>ADYVLAIDQGTTSSRAIVFDHSGEIYSTGQLEHDQIFPRAGWVEHNPEQIWNNVREVVGLALTRGNLTHEDIAAVGITNQRETAVVWDKTTGKPVYNAIVWQDTRTQKIVDELGGDEGAEKYKSIVGLPLATYFSGPKIKWILDNVEGAREKAEKGDLLFGNTDTWVLWNMTGGTEGGVHVTDVTNASRTMLMDLDTLSWREDIAADMGIPLSMLPDIRSSSEVYGHGRPRGLVPGVPIAGILGDQQAATFGQACFEVGQAKNTYGTGNFLLLNTGTEKVMSKNGLLTTVCYKIGDAPAVYALEGSIAVTGSLVQWLRDNLGMFEDAPDVEWLAGKVQDNGGAYFVPAFSGLFAPYWRPDARGALVGLTRYVNRNHIARAALEATAFQSREVVDAMNADSGVDLTELRVDGGM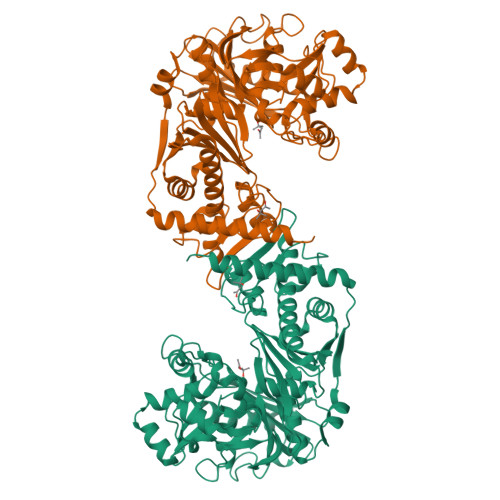VANELLMQFQADQLGVDVVRPKVAETTALGAAYAAGIAVGFWKGEQDVIDNWAEDKRWSPSMESGERERLYRNWKKAVTKTMEWVDEDVEQ[2x]> FNLDAEAPAVLSGPPGSFFGFSVEFYRPGTDGVSVLVGAPKANTSQPGVLQGGAVYLCPWGASPTQCTPIEFDSKGSRLLESSLSSSEGEEPVEYKSLQWFGATVRAHGSSILACAPLYSWRTEKEPLSDPVGTCYLSTDNFTRILEYAPCRSDFSWAAGQGYCQGGFSAEFTKTGRVVLGGPGSYFWQGQILSATQEQIAESYYPEYLINLVQGQLQTRQASSIYDDSYLGYSVAVGEFSGDDTEDFVAGVPKGNLTYGYVTILNGSDIRSLYNFSGEQMASYFGYAVAATDVNGDGLDDLLVGAPLLMDRTPDGRPQEVGRVYVYLQHPAGIEPTPTLTLTGHDEFGRFGSSLTPLGDLDQDGYNDVAIGAPFGGETQQGVVFVFPGGPGGLGSKPSQVLQPLWAASHTPDFFGSALRGGRDLDGNGYPDLIVGSFGVDKAVVYRGRPVV;> QTDENRCLKANAKSCGECIQAGPNCGWCTNSTFLQEGMPTSARCDDLEALKKKGCPPDDIENPRGSKDIKKNKNVTNRSKGTAEKLKPEDITQIQPQQLVLRLRSGEPQTFTLKFKRAEDYPIDLYYLMDLSYSMKDDLENVKSLGTDLMNEMRRITSDFRIGFGSFVEKTVMPYISTTPAKLRNPCTSE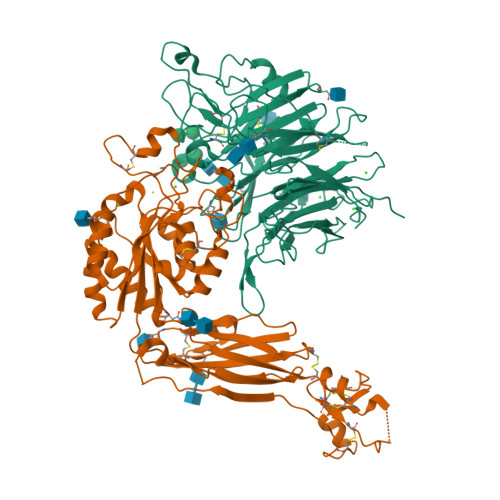QNCTTPFSYKNVLSLTNKGEVFNELVGKQRISGNLDSPEGGFDAIMQVAVCGSLIGWRNVTRLLVFSTDAGFHFAGDGKLGGIVLPNDGQCHLENNMYTMSHYYDYPSIAHLVQKLSENNIQTIFAVTEEFQPVYKELKNLIPKSAVGTLSANSSNVIQLIIDAYNSLSSEVILENGKLSEGVTISYKSYCKNGVNGTGENGRKCSNISIGDEVQFEISITSNKCPKKDSDSFKIRPLGFTEEVEVILQYICECE;> RGD>PCLTGPRTCKDLLDRGHFLSGWHTIYLPDCRPLTVLCDMDTDGGGWTVFQRRVDGSVDFYRDWATYKQGFGSRLGEFWLGNDNIHALTAQGTSELRTDLVDFEDNYQFAKYRSFKVADEAEKYNLVLGAFVEGSAGDSLTFHNNQSFSTKDQDNDLNTGNCAVMFQGAWWYKNCHTSNLNGRYLRGTHGSFANGINWKSGKGYNYSYKVS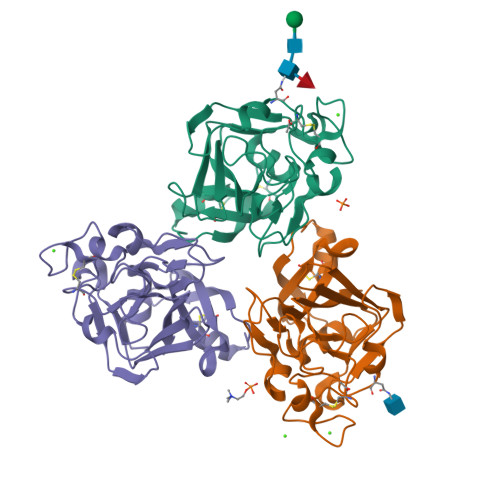EMKVRPA[3x]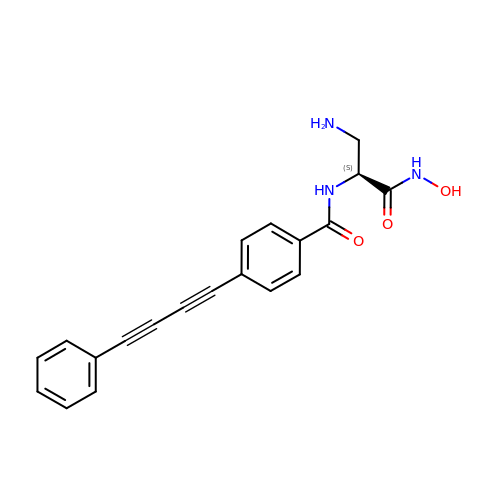N-[(2S)-3-amino-1-(hydroxyamino)-1-oxopropan-2-yl]-4-(4-phenylbuta-1,3-diyn-1-yl)benzamide | C20 H17 N3 O3 | RMTUQHBOIGEBSC-SFHVURJKSA-N> MSASNKGGYKTPRKENLMSIENLTNSEEESEDLNTAMVGNAVESQPKVTSRRSTRRPSPTKKYQAYQKESNGKGQEERIVVNYVEMSDERSSDAEDQEEEESIEESENAARPAAKDLHLIQSEYNVAGTSMFGFNTPKKRDAMALAALNATPCTPKTPKTPRLGVKTPDTKRKKSMDQPKTPAHVRTRVKKQIAKIVADSDEDFSGDESDFRPSDEESSSSSSSSDAGNSSDNDAADDEPKTPSRARRAIVV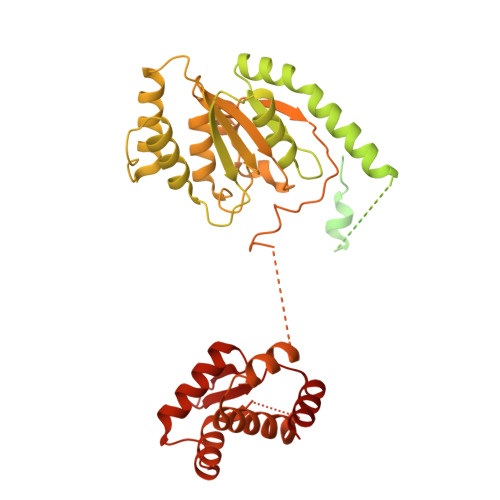PVLPKTPSAARLRQSARAKKSNEFVPESDGYFHSHASSKILTSDHTLDRLKNPRLAADRVFSLLSEIKTSAEHEGSINAIMEEYRSYFPKWMCILNEGFNILLYGLGSKHQLLQSFHREVLHKQTVLVVNGFFPSLTIKDMLDSITSDILDAGISPANPHEAVDMIEEEFALIPETHLFLIVHNLDGAMLRNVKAQAILSRLARIPNIHLLASIDHINTPLLWDQGKLCSFNFSWWDCTTMLPYTNETAFENSLLVQNSGELALSSMRSVFSSLTTNSRGIYMLIVKYQLKNKGNATYQGMPFRDLYSSCREAFLVSSDLALRAQLTEFLDHKLVKSKRSVDGSEQLTIPIDGALLQQFLEEQEKK> KTDVRWATFNIRYDNPQDSLNNWQYRKDRVCQFIKDHELDIVGMQEVLHNQFQDLRAGLPEYDGIGVGRDDGKTAGEYAPLFYRKDKYEVLDSNTFWLAENPDSVGMMGWDAVCVRIATWAKFKDKATGKIFMAVNTHFDHVGEEARRQSALLIIRKIKEIVGERPAVVTGDFNVTDASDAYETITTNEFVMKDAYKTAARVTGVD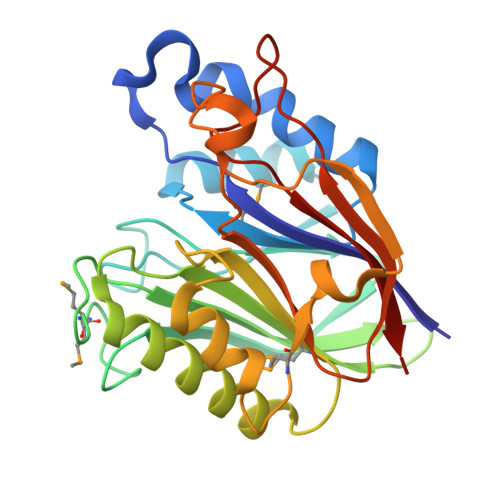YTFHDFARIPAEDCEKIDFIFVTPQVLVKSCEIPAEVPEALLSDHNPQLADLELEHHHHHH>[6x]PPGPPGPPGPPGPGPPGPPGPPGPPG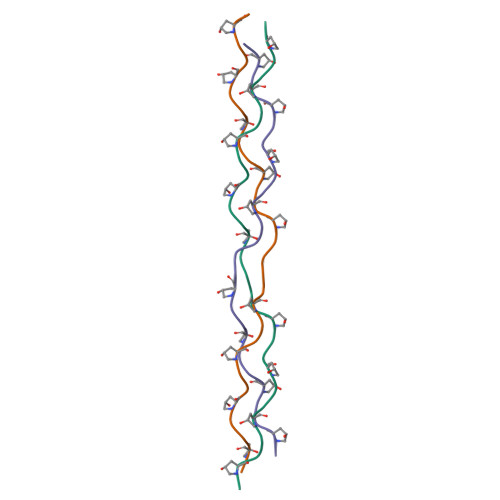PPG>GYTLWNDQIVKDEEVKIDKEDRGYQFGDGVYEVVKVYNGEMFTVNEHIDRLYASAEKIRITIPYTKDKFHQLLHELVEKNELNTGHIYFQVTRGTSPRAHQFPENTVKPVIIGYTKENPRPLENLEKGVKATFVEDIRWLRCDIKSLNLLGAVLAKQEAHEKGCYEAILHRNNTVTEGSSSNVFGIKD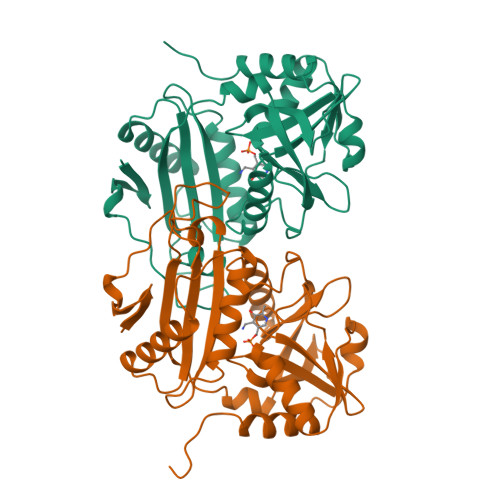GILYTHPANNMIAKGITRDVVIACANEINMPVKEIPFTTHEALKMDELFVTSTTSEITPVIEIDGKLIRDGKVGEWTRKLQKQFETKIPKPLHI[2x]> AAAAAAMTMMDMNFKYCHKIMKKHSKSFSYAFDLLPEDQRKAVWAIYAVCRKIDDSIDVYGDIQFLNQIKEDIQSIEKYPYEYHHFQSDRRIMMALQHVAQHKNIAFQSFYNLIDTVYKDQHFTMFETDAELFGACYGVAGTVGEVLTPILSDHETHQTYDVARRLGESLQLINILRDVGEDFENERIYFSKQRLKQYEVDIAEVYQNGVNNHYIDLWEYYAAIAEKDFRDVMDQIKVFSIEAQPIIELAARIYIEILDEVRQANYTLHERVFVEKRKKAKLFHEINSKYHR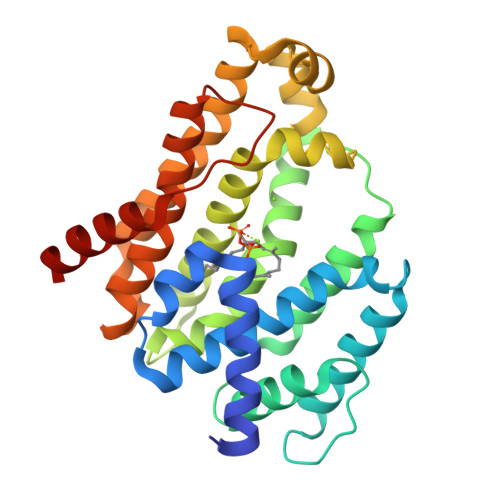I>[2x]GPGSNEFYLKTWSEWEKNGTPG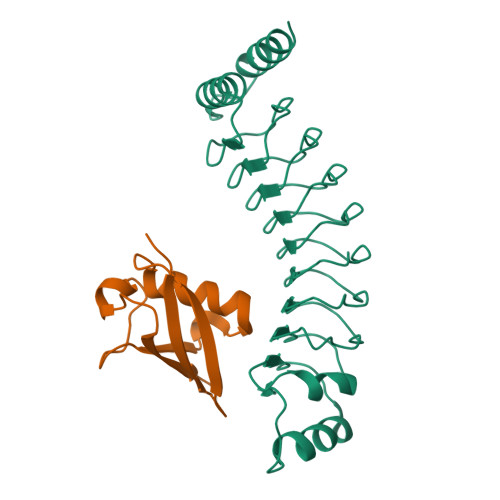EQRNIAFNRLKICLQNQEAELNLSELDLKTLPDLPPQITTLEIRKNLLTHLPDLPPMLKVIHAQFNQLESLPALPETLEELNAGDNKIKELPFLPENLTHLRVHNNRLHILPLLPPELKLLVVSGNRLDSIPPFPDKLEGLALANNFIEQLPELPFSMNRAVLMNNNLTTLPESVLRLAQNAFVNVAGNPLSGHTMRTLQQITTGPDYSGPRIFFSMG;>[2x]GPGSEFQDIRLWVSVEDAQMHTVTIWLTVRPDMTVASLKDMVFLDYGFPPVLQQWVIGQRLARDQETLHSHGVRQNGDSAYLYLLSARN> MINDMHPSLIKDKDIVDDVMLRSCKIIAMKVMPDKVMQVMVTVLMHDGVCEEMLLKWNLLDNRGMAIYKVLMEALCAKKDVKISTVGKVGPLGCDYINCVEISM

Here, we have developed a cell-free protein crystallization (CFPC) method, which involves direct protein crystallization using cell-free protein synthesis. We have succeeded in determining crystal structures of two types of proteins with high-resolution using CFPC. The polyhedra crystal (PhC) produced in insect cells by infection of cypovirus (cytoplasmic polyhedrosis virus, CPV) is one of the most highly studied in-cell protein crystals. The structure of crystalline inclusion protein A (CipA), a bacterial in-cell crystal, had not been previously reported.

Crystalline inclusion protein A (CipA), a hydrophobic protein of 104 amino acid residues, spontaneously forms crystalline aggregates in Photorhabdus luminescens, an entomopathogenic bacterium. Its native function is postulated to be involved in nematode symbiosis or pathogenesis. Since we found that twin crystals are formed when CipA is expressed in E. coli, we applied CFPC to CipA with the addition of twin crystal inhibitors during the crystallization process and succeeded in obtaining suitable crystals and determining the structure of CipA at a 2.11 Å resolution. X-ray diffraction experiments of the crystals showed that CipAC_CF crystallized in the presence of 3 v/v % 1,4-dioxane dramatically reduces the twin fraction to 0.10, with a resolution of 2.11 Å. The structure was determined by the molecular replacement method using the search model created by AF231 via ColabFold35. The structure of the CipA monomer consists of the N-terminal arm followed by three β-strands β1, β2, β3, α-helix, and β-strands β4 and β5. Except for the N-terminal arm, the globular domain is a typical oligonucleotide/oligosaccharide-binding (OB) fold. In the crystal lattice, the four α-helices from each monomer form a four-helix bundle around the crystallographic fourfold symmetry axis and exist as a tetramer. This tetramer is consistent with the results of PISA36 prediction of oligomeric states and is considered the basic unit of crystal growth. CipAC_CF forms a multilayer structure composed of the tetramers as the building blocks.> MMEKPEGLKLIDENGRRIDGRKKYELRPIKMEVGVLKNANG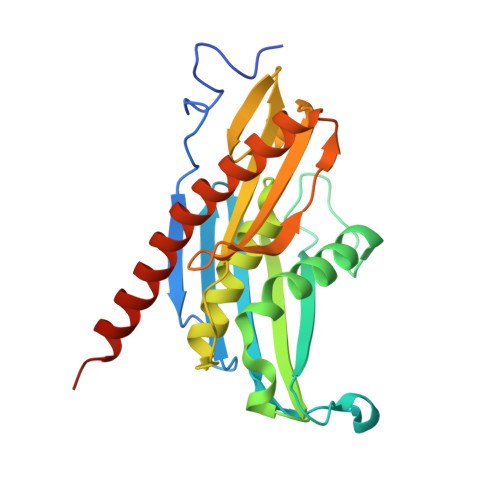SAYIEWGKNKIIAAVYGPRELHPKHLQRPDRAILRVRYNMAPFSVEERKKPGPDRRSIEISKVIKGALEPALILEMFPRTAIDVFIEVLQADAGTRVAGITAASLALADAGIPMRDLVAACAAGKIEGEIVLDLNKEEDNYGEADVPVAIMPLKNDITLLQMDGYLTKDEFIEAVKLAIKGAKAVYQKQREALKEKYLKIAQEVEGSE>MHSTTPISSLFSFTSPAVKRLLGWKQGDEEEKWAEKAVDSLVKKLKKKKGAMDELERALSCPGQPSKCVTIPRSLDGRLQVSHRKGLPHVIYCRVWRWPDLQSHHELKPLECCEFPFGSKQKEVCINPYHYRRVETPV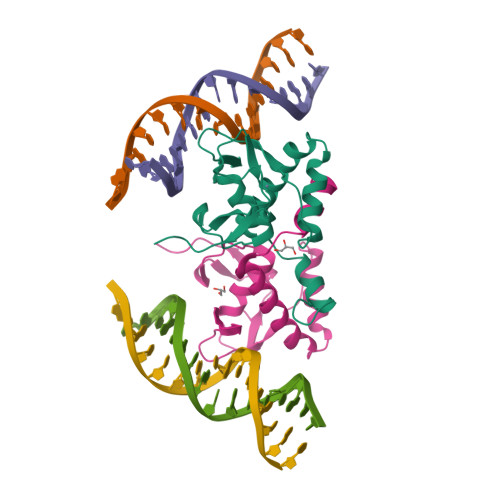LP[2x]Here, we introduce a close ortholog of MroUPO, a UPO gene from Marasmius wettsteinii (MweUPO-1), that has a similar reaction profile to MroUPO and for which we have set up a directed evolution platform based on tandem-yeast expression. As a member of the heme-thiolate-containing peroxidase superfamily, UPO activity is fueled simply by H2O2, which plays a dual role of oxygen donor and final electron acceptor. In general terms, long UPOs are monomeric proteins with a molecular weight of ∼44 kDa and with a strong preference toward small aromatic compounds due to their narrower and “carafe-shaped” heme channel (e.g., AaeUPO vide infra). By contrast, short UPOs are either dimeric or monomeric proteins with a molecular size of ∼26 kDa per monomer, harboring a wide open and symmetric cone-shaped channel (frustum) that dictates their preference for bulky substrates like steroids and long aliphatic compounds (a preference attributed to MroUPO, see below). Here we present a new dimeric short UPO that can be heterologously expressed at high levels in both S. cerevisiae and P. pastoris, an enzyme that shares its substrate profile, selectivity, and biochemical and overall structural characteristics with MroUPO.

High-quality large plate crystals were grown in 10–20% (v/v) PEG 4000/0.2 M (NH4)2SO4, and the crystals diffracted to a maximum resolution of 1.58 Å. The crystals belong to the P43212 space group, with two molecules per asymmetric unit. The electron density maps allowed the whole polypeptide chain to be modeled, from Ser1 to Leu236. The model contains the characteristic heme-thiolate prosthetic domain, the structural Mg2+ ion, and any remaining GlcNAc units attached to the Asn35, Asn122, and Asn143 N-glycosylation sites. The asymmetric unit of the MweUPO-1 crystal structure consists of two identical polypeptide chains that are arranged in a homodimer. The monomer is mostly helical, and it is comprised of 11 α-helices and two short β-strands. These monomers are covalently linked through an intermolecular disulfide bridge between Cys227 of both polypeptides, and many hydrophobic contacts are formed among the Val62, Leu65, Ile230, and Leu232 residues in each chain. Interestingly, there is a clear density where a second water molecule establishes a polar link to this distal water molecule, putatively mimicking the early ferric-peroxo complex (“pre-compound 0”) formed in the first step of the postulated catalytic cycle of UPOs. The heme access cavity is a 17 Å long, deep funnel with a wide irregularly shaped entrance that reduces to a narrow base close to the heme group. Another interesting feature of the MweUPO-1 heme channel is the absolute lack of ordered water molecules, even in the ligand-free crystals.

>[2x]AVDFSAHPWKAPGPNDSRGPCPGLNTLANHGFLPRNGRNISVPMIVKAGFEGYNVQSDILILAGKVGMLTSREADTISLEDLKLHGTIEHDASLSREDVAIGDNLHFNEAIFTTLANSNPGADVYNISSAAQVQHDRLADSVARNPNVTNTDLTATIRSSESAFYLTVMSAGDPLRGEAPKKFVNVFFQEERMPIKEGWKRSTTPINLPLLGPIIDRITELSDWKPTGDNCGAIVLGPGL Here, we study DHPS-3-dehydrogenase from Cupriavidus pinatubonensis (CpHpsN), a bacterium capable of utilizing DHPS as a sole carbon source. Kinetic analysis of CpHpsN reveals a strict preference for R-DHPS, catalyzing its 4-electron oxidation to R-SL, with high specificity for NAD+ over NADP+. CpHpsN forms a domain-swapped tight dimer with 28% of surface area buried at the dimer interface, with the interface featuring extensive hydrophobic and hydrogen-bond interactions. Domain 4 lies at the C-terminus and contributes to the active site and is also involved in dimerization through a metal binding site. Coordination of Zn2+ involves three residues from one monomer and one residue (His411*; * denotes the other monomer in the dimer) from the other monomer (Fig. 5 and S7†), showing that the enzyme forms an obligate dimer.

Crystals of the CpHpsN·Zn2+·NADH complex were obtained by soaking CpHpsN·Zn2+ crystals with NADH and diffracted to 2.24 Å. Attempts to soak the CpHpsN·Zn2+ crystals with high concentrations of NADH/NAD+, and SL or DHPS were unsuccessful to obtain a substrate or product bound complex. CpHpsN structures in both space groups contain a dimer in the asymmetric unit. No activity was detected for the D352A mutant of CpHpsN, most likely due to the inability to form a productive zinc-coordination complex with substrate. The 3D structure of the CpHpsN D352A mutant in complex with Zn2+ and NAD+ was solved and refined to 2.23 Å resolution and is essentially identical to the CpHpsN·Zn2+·NADH structure in the ‘open’ conformation (Fig. S12a–c†).

>[2x]GMISYLKKAEKTPQTETATAQKVVTEMLAEIQARGKDAVRQYAKQLDGWSGDIVLTPDQIREQTKDVPAGVRADIDFAIRQVTDFALAQRESLKEFSVELHPGVTAGQRVLPVNVVGCYAPAGRYAHIASAYMGVATAKAAGVKTVVACSSPFRGQGIHPHVLYAFQAAGADVIMALGGVQAIASMAYGLFTGKPADVVVGPGNKFVAEAKRSLYGQVGIDVFAGPSEVAVIADETADPAIVASDLVGQAEHGHESPAWLFTTSRDLADRVMALVPELIAKLPPTARDAATAAWRDYGEVILCGTREEVVEISDRYASEHLEVHTADLDWWLANLTCYGSLFLGEETTVAFGDKTSGPNHVLPTKGAARYSGGLSVHKFMKTLTWQQMTREATRQIGQVTARISRLEGMEAHARTADDRMAKYFPNASFEMGTPVEV>[2x]MVEKFVGTWKIADSHNFGEYLKAIGAPKELSDGGDATTPTLYISQKDGDKMTVKIEQGPPTFLDTQVKFKLGEEFDEFPS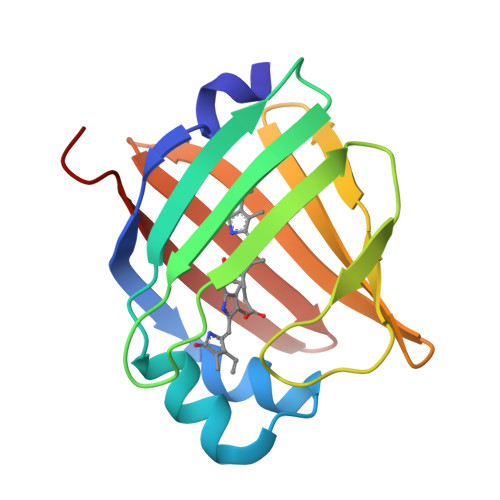DRRKGVKSVVNLVGEKLVYVQKWDGKETTYVREIKDGKLVVTLTMGDVVAVRSYRRATE> NHPMLMNL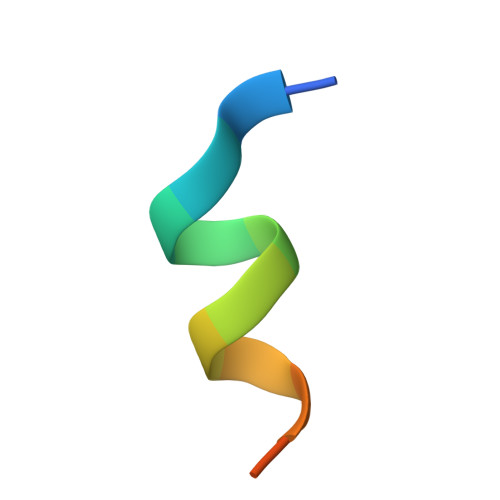LKDNPA> GPMNPGPLELQLGDIFIAVKTTWAFHRSRLDLLLDTWVSRIRQQTFIFTDSPDERLQERLGPHLVVTQCSAEHSHPALSCKMAAEFDAFLVSGLRWFCHVDDDNYVNPKALLQLLKTFPQDRDVYVGKPSLNRPIHASELQSKQRTKLVRFWFATGGAGFCINRQLALKMVPWASGSHFVDTSALIRLPDDCTVGYIIECKLGGRLQPSPLFHSHLETLQLLGA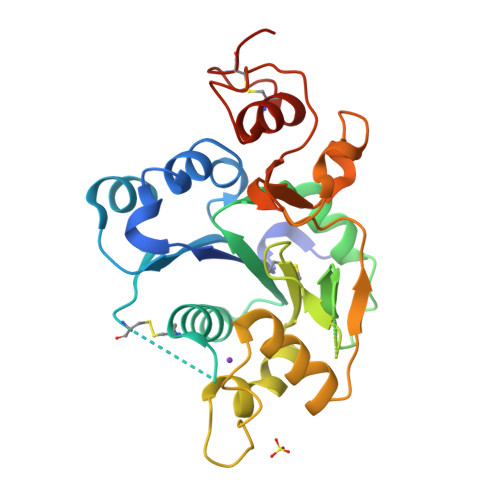AQLPEQVTLSYGVFEGKLNVIKLPGPFSHEEDPSRFRSLHCLLYPDTPWCPLLAAP> HDVGEVNGDALSAQEYQNLVEEYTEVIKLSRGVTALNDEQTNQVRDEVWRSYVNNKLVEKEAKALGLTVSAAEIQDILKAGVHPLLQQTPFRNPQTGAFDKDMLNKFLVDYAKMNESQMPAQYAEQYNNMYKYWSFIQKTLVQSRLAEKYQALVAKALLSNPVEAQDAFDARVNQYDLLMAAVPYSSIVDSTIVVKESELKDLYNKKKEQFKQYQESRDIKYIDVQVTASAEDRAAIQQEVDEATAQLATTTDDYTSFIRSVGSEAPYVDLFYNKTAFPSDVVARLDSASVGSVYGPYYNGADNTINSFKVVAKTAAADSIEFRQIQVFAEDALKTKALADSIYTAIKGGANFADLAKKYGQTGETNWMSSAQYEGAQIDGDNLKFISAINNTGVNEVVNLPLGQANVILQVTNKKAVKDKYKVAVVKREVEFSKETYNRAYNDFSQFIAANPTAEKMIANAEEAGYKLLDRRDLYSSEHTIGGVRGTKEALRWAFSAKPGDVSGLYECGESDHMVAVALVGVTP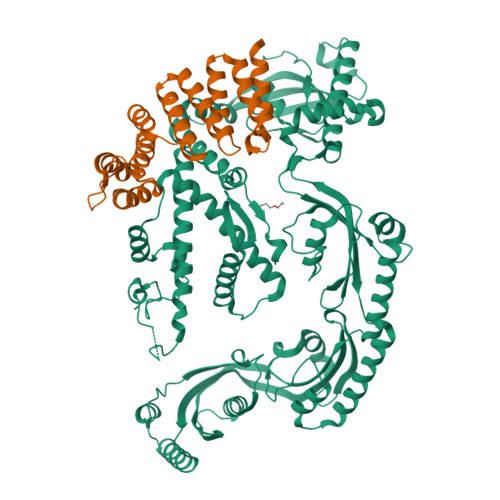EGYRPLKAVQDQLRAEIVKDKKAEKIMADMKAANATSLDQYKAMSGAVSDSLKLVTFAAPAYVSALRSSEPLVGAYASVAEMNKLSAPIKGNAGVFVLQMYGKDKLSDTFNAKDEEATLANMHARFASRLMNDLYLKGKVKDTRYLFF;> PREEKAQAALFKGQEYFEQDAYEQALNGDSIGYVGFLKVADEYSGTKAANLAKAYAGICYAQLGKYDEAVKMLDGFNGGDQMVAPAILGATGNCYAQLGQLDKAASTLLSAADKADNNSLSPIFLMQAGEILVKQGKYDDAVNAYTKIKDKYFQSYQAMDIDKYIEQAKLMKK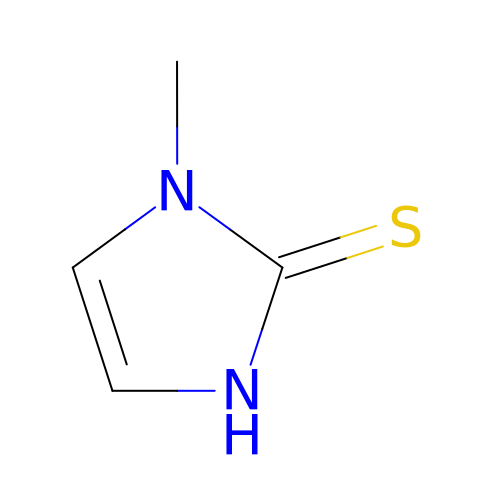1-METHYL-1,3-DIHYDRO-2H-IMIDAZOLE-2-THIONE | C4 H6 N2 S | PMRYVIKBURPHAH-UHFFFAOYSA-N> AEQSSSEIKIVRDEYGMPHIYANDTWHLFYGYGYVVAQDRLFQMEMARRSTQGTVAEVLGKDFVKFDKDIRRNYWPDAIRAQIAALSPEDMSILQGYADGMNAWIDKVNTNPETLLPKQFNTFGFTPKRWEPFDVAMIFVGTMANRFSDSTSEIDNLALLTALKDKYGVSQGMAVFNQLKWLVNPSAPTTIAVQESNYPLKFNQQNSQT;> SNMWVIGKSKAQDAKAIMVNGPQAGWYAPAYTYGIGLHGAGYDVTGNTPFAYPGLVFGHNGVISWGSTAGFGDDVDIFAERLSAEKPGYYLHNGKWVKMLSREETITVKNGQAETFTVWRTVHGNILQTDQTTQTAYAKSRAWDGKELASLLAWTHQMKAKNWQEWTQQAAKQALTINWYYADVNGNIGYVHTGAYPDRQSG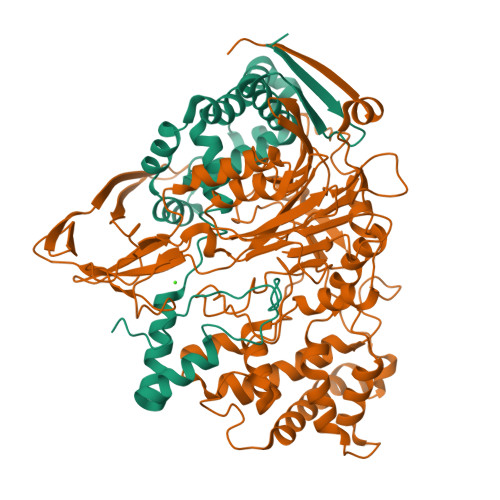HDPRLPVPGTGKWDWKGLLPFEMNPKVYNPQSGYIANWNNSPQKDYPASDLFAFLWGGADRVTEIDRLLEQKPRLTADQAWDVIRQTSRQDLNLRLFLPTLQAATSGLTQSDPRRQLVETLTRWDGINLLNDDGKTWQQPGSAILNVWLTSMLKRTVVAAVPMPFDKWYSASGYETTQDGPTGSLNISVGAKILYEAVQGDKSPIPQAVDLFAGKPQQEVVLAALEDTWETLSKRYGNNVSNWKTPAMALTFRANNFFGVPQAAAEETRHQAEYQNRGTENDMIVFSPTTSDRPVLAWDVVAPGQSGFIAPDGTVDKHYEDQLKMYENFGRKSLWLTKQDVEAHKESQEVLHVQR>SMKDELVVFSLPNLSSPFEVQLQKVAVETSKKLEIKLQVLDGQSSSTKQASDLENAITRGAKGIIISPNDVNAISGAVEEIIKEKIPAATLDRKVESSKPVPHFGANNYTGGQEVAKAVKAKYPNGAKIILLTGQPGSTSNIERTKGIRDELAAGGDKYKIVVDQTGNWLRSEGLRIIESVLPTLKEKPEVIISANDDMALGAIEALRSQGLKAGDILVTGFDSTPEALARVKDGWLYLTADQRPSFAVSTALEQVVGNIRESKEVSG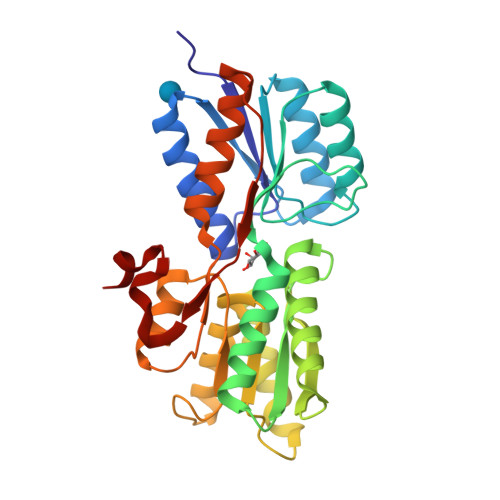ADYPPKIILKDNLQEAERFAEISE[2x]>[2x]MQFPQLDPATLAAFSAAFRGELIWPSDADYDEARRIWNGTIDRRPALIARCTSTPDVVAAVSFARKSGLLVAVRGGGHSMAGHSVCDGGIVIDLSLMNSIKVSRRLRRARAQGGCLLGAFDTATQAH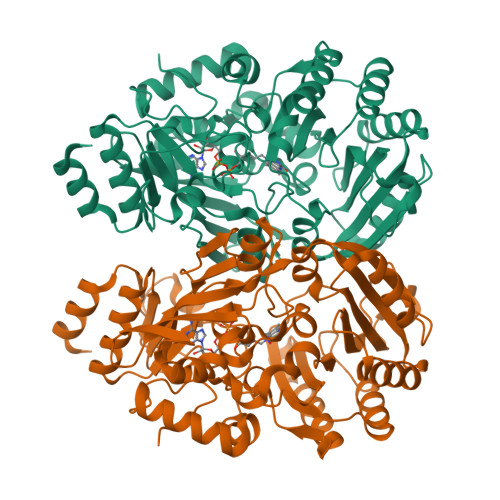MLATPAGVVSTTGLGGLVLGGGFGWLSRKYGLSIDNLTSVEIVTADGGVLTASDTENPDLFWAVRGGGGNFGVVTAFEFDLHRVGPVRFASTYYSLDEGPQVIRAWRDHMATAPDELTWALYLRLAPPLPELPADMHGKPVICAMSCWIGDPHEGERQLESILHAGKPHGLTKATLPYRALQAYSFPGAVVPDRIYTKSGYLNELSDEATDTVLEHAADIASPFTQLELLYLGGAVARVPDDATAYPNRQSPFVTNLAAAWMDPTEDARHTAWAREGYRALAGHLSGGYVNFMNPGEADRTREAYGAAKFERLQGVKAKYDPTNLFRLNQNIPPSSP> MQTEHVILLNAQGVPTGTL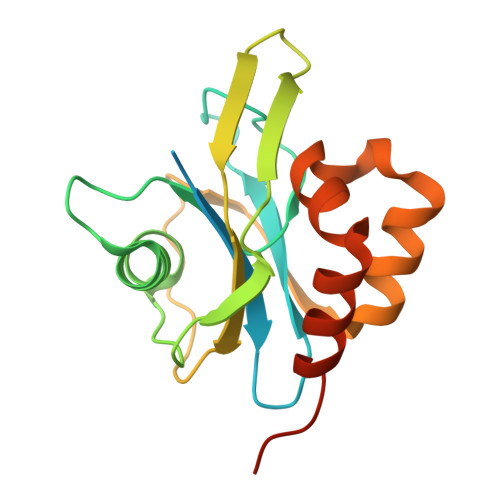EKYAAHTADTRLHLAFSSWLFNAKGQLLVTRRALSKKAWPGVWTNSVCGHPQLGESNEDAVIRRCRYELGVEITPPESIYPDFRARATDPSGIVENEVCPVFAARTTSALQINDDEVMDYQWCDLADVLHGIDATPWAFSPWMVMQATNREARKRLSAFTQLKLEHHHHHH> MEWSQIFHDITTKHDFKAMHDFLEKEYS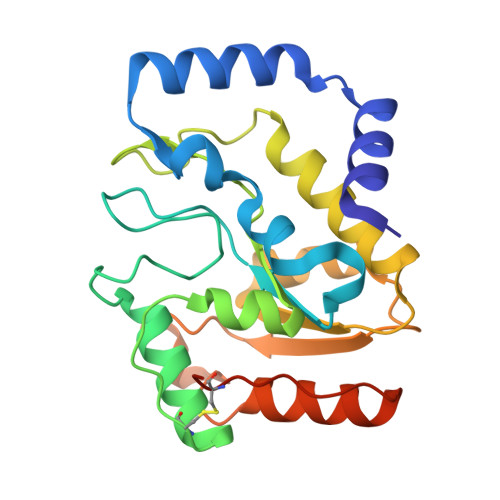TAIVYPDRENIYQAFDLTPFENIKVVILGQDPYHGPNQAHGLAFSVQPNAKFPPSLRNMYKELADDIGCVRQTPHLQDWAREGVLLLNTVLTVRQGEANSHRDIGWETFTDEIIKAVSDYKEHVVFILWGKPAQQKIKLIDTSKHCIIKSVHPSPLSAYRGFFGSKPYSKANTYLESVGKSPINWCESEALEHHHHHH GABARAPL2 (also called GATE-16) belongs to the GABARAP subfamily of Atg8 proteins. Like other Atg8 proteins, GABARAPL2 is comprised of an N-terminal helical extension preceding four β-sheets in a ubiquitin-like β-grasp fold. This fold forms the LIR docking site (LDS), consisting of hydrophobic pocket 1 (HP1) and hydrophobic pocket 2 (HP2). Once anchored, Atg8 proteins recognize autophagy receptors and adaptors by their canonical LIR motif, a small motif comprising Θ0-X 1-X 2-Γ3, where Θ represents an aromatic residue (W/F/Y), Γ an aliphatic residue (L/V/I) and X any amino acid.

In this work, we solved the apo structure of GABARAPL2 to 1.9 Å resolution in a new crystal form in an attempt to co-crystallize it with an LIR peptide. The structure reported here shares the same P21 space group as the published structure, but showed a different monoclinic angle and is not twinned. We collected diffraction data from 13 crystals that diffracted to resolutions within the range 2–3 Å, with the best diffracting crystal, with dimensions of approximately 5 × 50 × 400 µm, diffracting to 1.9 Å resolution. All data sets belonged to space group P21 with similar unit-cell dimensions, and the best diffracting crystal, which we discuss here, had unit-cell dimensions a = 28.4, b = 58.7, c = 69.0 Å and a monoclinic angle of 98.3°. Despite sharing similar unit-cell dimensions, with the b and c axes permuted, the structure that we present does not show a twinned crystal pathology, which is likely to be due to the change in the monoclinic angle. In the new crystal, there is a change in the orientation of Arg28 that allows the formation of a bidentate salt bridge to Glu12 from its +1/2, −z symmetry mate. As Phe117 of GABARAPL2 forms a dominant crystal contact that blocks LIR peptide binding, this suggests that future co-crystallization studies should remove this residue to enable new crystal forms that permit LIR peptide binding.

>[2x]GAMSMKWMFKEDHSLEHRCVESAKIRAKYPDRVPVIVEKVSGSQIVDIDKRKYLVPSDITVAQFMWIIRKRIQLPSEKAIFLFVDKTVPQSSLTMGQLYEKEKDEDGFLYVAYSGENTFGF Spleen tyrosine kinase (Syk) is a non-receptor tyrosine kinase expressed broadly in the hematopoietic lineage and an essential component in leukocyte signal transduction. Syk binds to and is activated by immunoreceptors Fc-epsilon (FcεR), Fc-gamma (FcγR), or the B-cell receptor (BCR) in the appropriate cellular context. Syk therefore has a central role in antibody-dependent immune cell activation and may mediate, at least in part, the pathophysiological mechanisms that underlie numerous instances of autoimmune disease. Syk kinase inhibitors have emerged as promising therapeutic agents for the treatment of autoimmune diseases such as RA.

Here we describe the identification of a potent, moderately selective, and orally bioavailable small molecule Syk kinase inhibitor based on a novel triazolopyridine core. Structure-based guided optimization of a triazolopyridine screening hit led to the identification of CC-509, an active and reversible inhibitor of Syk enzyme with an IC50 value = 0.026 +/- 0.006 μM (n = 8) and a Ki of 18 nM. Based on enzyme kinetics, CC-509 is a mixed competitive inhibitor with respect to the Syk ATP binding site. Consistent with this mode of inhibition, the co-crystal structure of CC-509 in Syk shows the inhibitor bound primarily in the ATP binding pocket via two hydrogen bonds with hinge residue Alanine 451. Based on its activity in this panel of kinases, the calculated Gini score (a metric for kinase selectivity) of 0.53 for CC-509 indicates the compound is considered moderately selective. For comparison, R406 also blocked Y525/526 phosphorylation at comparable potency (IC50 value = 0.72 ± 0.66 μM). This data indicate CC-509 is a cell-permeable and potent inhibitor of cellular Syk kinase activity. CC-509 inhibits FcεR-, FcγR-, and BCR-mediated signaling in disease-relevant and primary cell types. CC-509 was the result of an optimization campaign toward improved selectivity with respect to the overall kinome and away from specific kinase targets such as KDR and Jak that likely contributed to aspects of the fostamatinib side-effect profile. Importantly, CC-509 was successfully optimized to improve overall kinase selectivity and activity against KDR and Jak, and has a clearly differentiated profile when compared to R406. In conclusion, we describe a novel triazolopyridine-based Syk kinase inhibitor, CC-509, with potent cellular activity in FcR-dependent systems, favorable PK properties, and efficacy in models of inflammatory disease and arthritis.

> MDTEVYESPYADPEEIRPKEVYLDRKLLTLEDKELGSGNFGTVKKGYYQMKKVVKTVAVKILKNEANDPALKDELLAEANVMQQLDNPYIVRMIGICEAESWMLVMEMAELGPLNKYLQQNRHVKDKNIIELVHQVSMGMKYLEESNFVHRDLAARNVLLVTQHYAKISDFGLSKALRADENYYKAQTHGKWPVKWYAPECINYYKFSSKSDVWSFGVLMWEAFSYGQKPYRGMKGSEVTAMLEKGERMGCPAGCPREMYDLMNLCWTYDVENRPGFAAVELRLRNYYYDVVNHHHHHH> MEDGAQMRVVAFGDQTYDCSEAVSQLLRVRDDAIVVDFLERAPAVLKAELARLSSEQQEETPRFATLAELVPRYRAGTLNPAVSQALTCIAQLGLFIRQHSSGQEAYPTAHDSCITGVATGALTAVAVGSASSVTALVPLALHTVAVAVRLGARAWEIGSCLADARRGANGRYASWTSAVGGISPQDLQDRISAYTAEQALASVSVPYLSAAVGPGQSSVSAAPVILDAFLSTLLRPLTTTRLPITAPYHAPHLFTAKDVQHVTDCLPPSEAWPTVRIPIISFSRDEAVSRGASFPAAMSEAVRDCLIRPIALDRMAVSIANHARDLGKDSVLPSPIALSFSDKLGP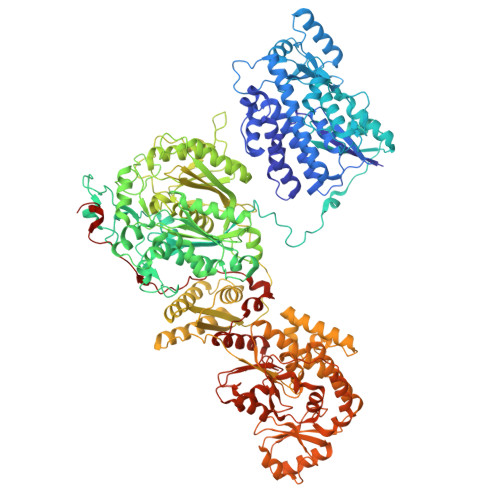QVNSHLPGAKAPTPELTSKSIPSAIGAEQQPMAKSPIAILAASGRFPQSSSMDQFWDVLINGVDTHELVPPTRWNAATHVSEDPKAKNVSGTGFGCWLHEAGEFDAAYFNMSPREAPQVDPAQRLALLTATEALEQAGVVPNRTSSTQKNRVGVWYGATSNDWMETNSAQNVDTYFIPGGNRAFIPGRVNYFHKFSGPSYTIDTACSSSLAALHMACNALWRGEVDTAIVGGTNVLTNPDMTAGLDAGHFLSRSGNCKTFDDEADGYCRGEAVVTLILKRLPDAQADKDPIQASILGIATNHSAEAASITRPHAGAQQDLFQQVLTETGLTANDISVCEMHGTGTQAGDSGETTSVVETLAPLNRSGSAVRTTPLYIGAVKSNVGHAESAAGVSSLAKILLMLKHSKIPPHVGIKTKLNHRLPDLAARNTHIARSEVPWPRPKNGKRRVLLNNFSAAGGNTCLVLEDAPEPEDSQEVDPREHHIVALSAKTPDSMVNNLTNMITWIDKHSGDSLATLPQLSYTTTARRVHHRHRAVATGTDLLQIRSSLQEQLDRRVSGERSIPHPPNGPSFVLAFTGQGSAFAGMGVDLYKRFASFRSDIARYDQICEGMSLPSIKAMFEDEKVFSTASPTLQQLTHVCFQMALYRLWKSLGVQAKAVVGHALGEYAALYAAGVLSQSDTLYLVGRRAQLMEKHLSQGTHAMLAVRAKEEAIVAAIDGPPGEAYEFSCRNGEQRNVLGGTVAQIQAAKAALEAKKIRCQYLDTPMAFHTGQVDPILPELLQVAAACSIQDPQIPVISPAYGKVIRSAKDFQPEYFTHHCRSSVNMVDALQSAVEEGLLDKNVIGLEIGPGPVVTQFVKEAVGTTMQTFASINKDKDTWQLMTQALAKFYLAGASVEWSRYHEDFPGAQKVLELPAYGWALKNYWLQYVNDWSLRKGDPAVVVAASAAALEHHHHHH>[180x]SKVFNTQTFDIYSTEKDVVSLRDFANDKDTLAYKR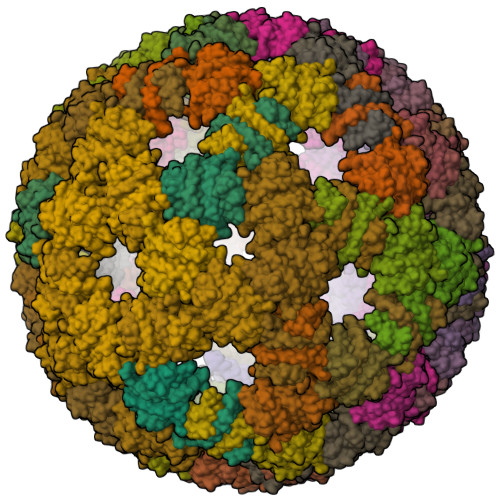LAPKRTKDSPGMAKSELKITRVDPTTGVLIGIVNVSSSIRADATAADKTALMAIITAAQADGAWTELVTDQRLPLATV> MPSKKKKYNARFPPARIKKIMQTDEEIGKVAAAVPVIISRALELFLESLLKKACQVTQSRNAKTMTTSHLKQCIE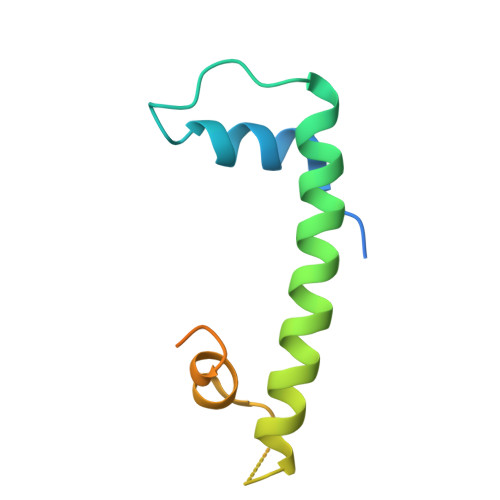LEGDPAANKARKEAELAAATAEQ(2~{S})-2-[[(4~{S})-4-azanyl-5-oxidanyl-5-oxidanylidene-pentanoyl]amino]pentanedioic 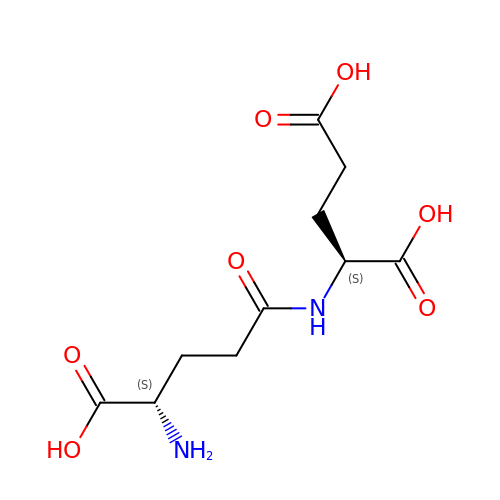acid | C10 H16 N2 O7 | OWQDWQKWSLFFFR-WDSKDSINSA-N CENP-E is essential for the alignment of chromosomes in metaphase. CENP-E specifically associates with unattached kinetochores to facilitate chromosome congression, interacting with BubR1 at the kinetochore through its C-terminal region (2091-2358). Our work reveals that CENP-E is recruited to unattached kinetochores through at least 2 pathways: a BubR1-dependent pathway involving the domain 2055-2358 and a pathway dependent on the outer corona and Dynein involving domain 2452-2598. We provide a structural model of the entire CENP-E kinetochore targeting domain combining X-ray crystallography and Alphafold2.

Next, we sought to determine the structure of this minimal corona-targeting domain. This domain contains a highly conserved region from Xenopus to humans that is predicted unstructured and flanked by two predicted α-helices. We therefore recombinantly expressed and purified CENP-E2452-2598. Using this approach, we found that CENP-E2452-2598 forms a dimer. We obtained protein crystals that diffracted anisotropically with resolution limits between 2.14 Å and 2.71 Å. Structural determination revealed a parallel dimeric coiled-coil in which only the first helical region of the construct was observed in electron density, likely because the construct underwent C-terminal degradation during crystallization. The resultant structural model corresponds to amino acids K2454 to S2506 of CENP-E. The structure reveals a tight left-handed coiled-coil in which the hydrophobic heptad interface involves aromatic stacking of F2478 residues. Surrounding interactions that stabilize the coiled-coil include salt bridges between the E2470 and K2471 side chains. The dimeric structure is consistent with the behaviour of CENP-E2452-2598 in solution, and is supported by previous data indicating this region mediates dimerization of the kinetochore-targeting domain of CENP-E2055-260819. The structure we determined is part of the coiled-coil on the N-terminal side of the loop and the conserved patch (highlighted in yellow). Overall, the CENP-E conserved patch and flanking helical coiled-coils are essential for outer corona targeting.

>GPSPYKEEIEDLKMKLVKIDLEKMKNAKEFEKEISATKATVEYQKEVIRLLRENLRRSQQAQDTSVISEHTDPQPSNKPLTCGGGSGIVQNTKALILKSEHIRLEKEISKLKQQNEQLIKQKNELLSNNQHLSNEVKTWKERTLKREAHK[2x]2-({4'-pentyl-3'-[(Z)-2-(pyridin-2-yl)ethenyl][1,1'-biphenyl]-4-yl}sulfonyl)ethan-1-ol 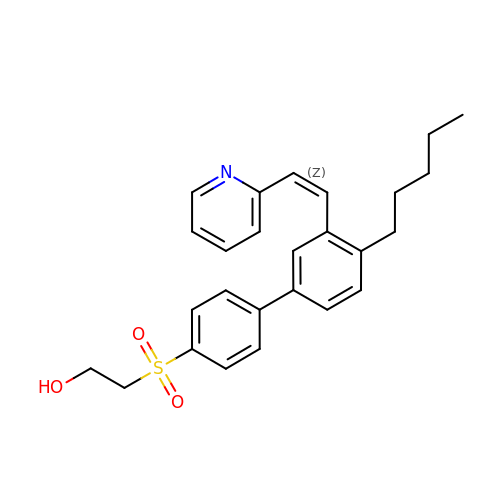| C26 H29 N O3 S | CNGQPWUWCYALEW-KAMYIIQDSA-N>[3x]AHCIGITDRDFIEGVHGGTWVSATLEQDKCVTVMAPDKPSLDISLETVAIDGPAEARKVCYSAVLTNVKINDKCPSTGEAHLEEENEGDNACKRTYSDRGWGNGCGLFGKGSIVACAKFTCAKSMSLFEVDQTKIQYVIRAQLHVGAKQENWNTDIKTLKFDALSGSQEAEFTGYGRA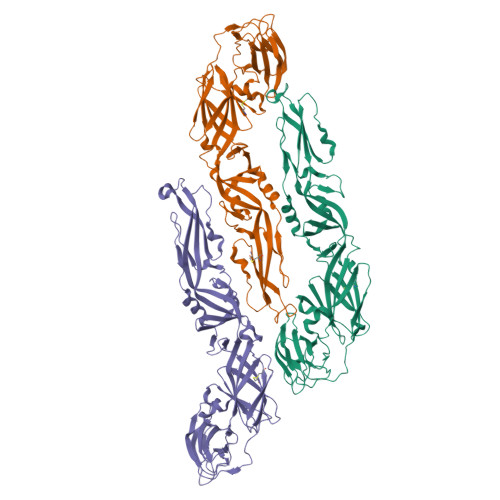TLECQVQTAVDFSNSYIAEMEKESWIVDKQWAQDLTLPWQSGSGGVWREMHHLVEFEPPHAATIKVLALGNQEGSLKTALTGAMRVTKDTNNSKLYKLHGGHVACRVKLSALTLKGTSYKMCTDKMSFVKNPTDTGHGTAVMQVKVPKGAPCRIPVMVADDLTAAVNKGILVTVNPIASTNDDEVLIEVNPPFGDSYIIVGRGDSRLTYQWHK>MAVPETRPNHTIYINNLNEKIKKDELKKSLHAIFSRFGQILDILVSRSLKMRGQAFVIFKEVSSATNALRSMQGFPFYDKPMRIQY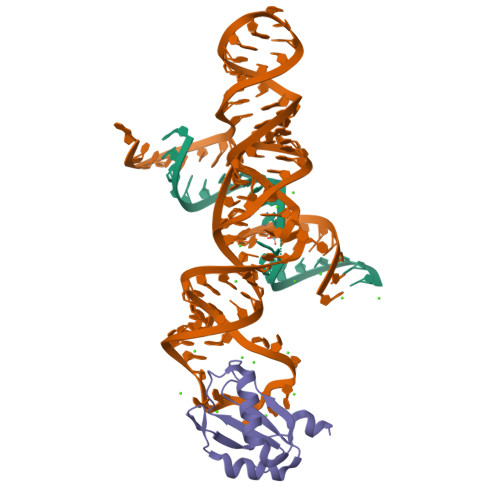AKTDSDIIAKMKGT[2x]2-{4-[2-ACETYLAMINO-2-(1-BIPHENYL-4-YLMETHYL-2-OXO-AZEPAN-3-YLCARBAMOYL)-ETHYL]-2-CARBOXY-PHENYL}-MALONIC ACID | C34 H35 N3 O9 | 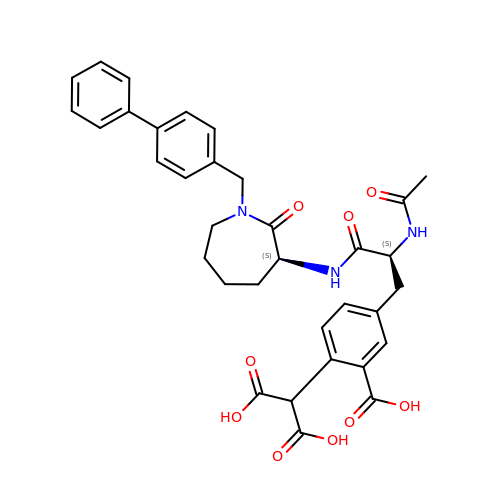CGOGPQNYHFBUEF-NSOVKSMOSA-N>MAHHHHHHMLELPPVASLKGKSITSAEQFSRADIYALIHLASAMQRKIDAGEVLNLLQGRIMTPLFFEDSSRTFSSFCAAMIRLGGSVVNFKVEASSINKGETLADTIRTLDSYSDVLVMRHPRQDAIEEALSVAQHPILNAGN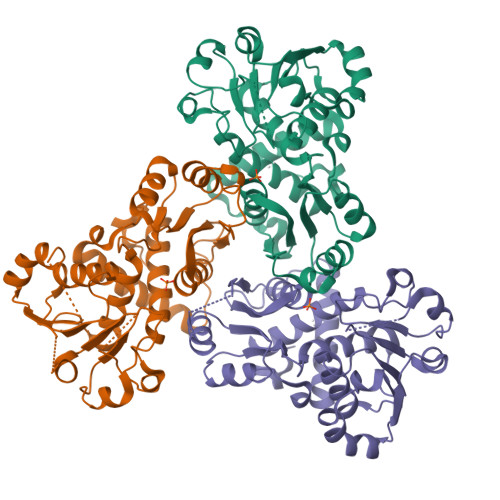GAGEHPTQALLDTLTIHSELGSVDGITIALIGDLKMGRTVHSLLKLLVRNFSIKCVFLVAPDALQMPQDVLEPLQHEIATKGVIIHRTHALTDEVMQKSDVLYTTRLQKERFMASTSDDAAALQSFAAKADITIDAARMRLAKEKMIVMHPLPRNDELSTTVDADPRAAYFRQMRYGMFMRMAILWSVLA[6x]> QGHMSNFLAEQYERDRKAIINCCFSRPDHKTGEPPNNYITHVRIIEDSKFPSSRPPPDSKLENKKKRLLILSAKPNNAKLIQIHKARENSDGSFQIGRTWQLTELVRVEK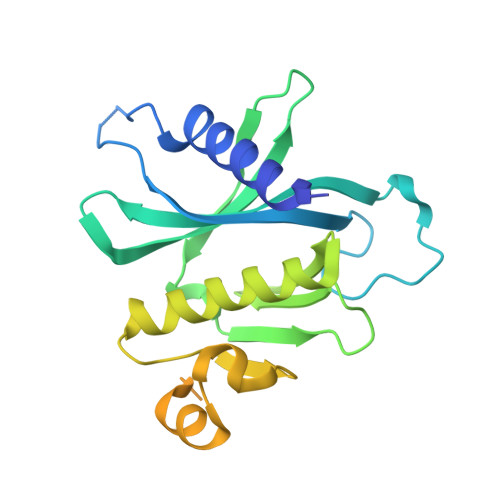DLEISEGFILTMSKKYYWETNSAKERTVFIKSLITLYIQTFEGHVPELVNWDLSLFYLDERSYQRAVITNRPGSVSPIKSPTSNFTTNTTQSVGSVPFSAPTERTRRSETESVNPVSTPASVEYHAGMKSLNKAPYSSNS>[2x]RKSKAELQSEERKRIDELIESGKEEGMKIDLIDGKGRGVIATKQFSRGDFVVEYHGDLIEITDAKKREALYAQDPSTGCYMYYFQYLSKTY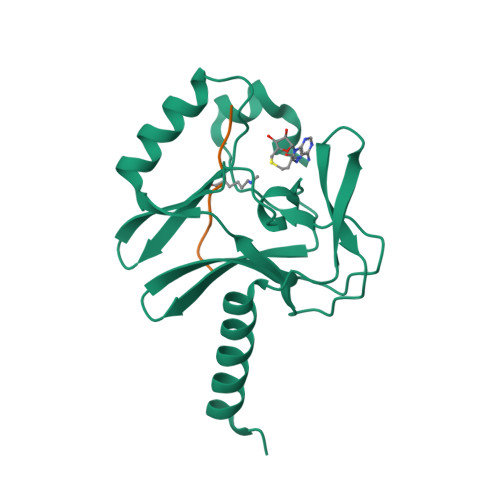CVDATRETNRLGRLINHSKCGNCQTKLHDIDGVPHLILIASRDIAAGEELLYDYGDRSKASIEAHPWLKH;>RHRKVLRDNY[2x]>SNAMTQAFSRVRFIMTQPSHPGNVGSAARAIKTMGFGELVLVAPRFPDMTAQPEAVALASGALDVLERAAVHDTLEEALAPVTLAFALTTRVRDLGPPPCDIREAAGLARRHLDDTEAGVVAIVLGTERAGLTNAQIELCHRICHIPANPQYSSLNV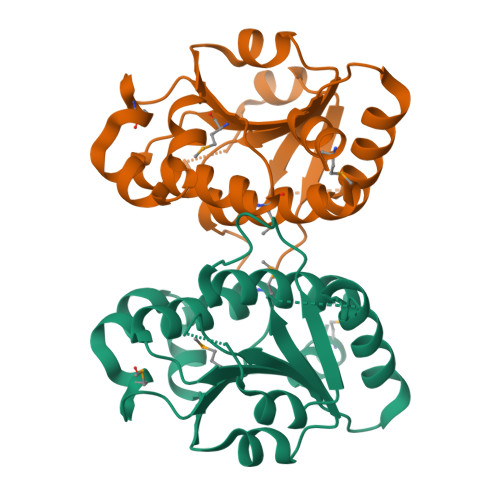AQALQLAAWELRYALL[3x]>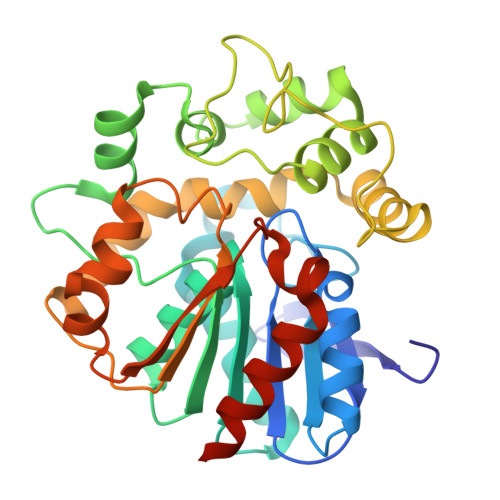 MEEIEHRTVEVNGIKMHVAEKGEGPVVLFLHGFPELWYSWRHQILALSSRGYRAVAPDLRGYGDTEAPVSISSYTGFHIVGDLIALIDLLGVDQVFLVAHDWGAIIGWYLCTFHPDRVKAYVCLSVPLLHRDPNIRTVDAMRAMYGDDYYICRFQKPGEMEAQMAEVGTEYVLKNILTTRKPGPPIFPKGEYGTGFNPDMPNSLPSWLTQDDLAYYVSKYEKTGFTGPLNYYRNMNLNWELTAPWSGGKIQVPVKFITGELDWVYTSLNMKEYIHGGGFKQDVPNLEEVIVQKNVAHFNNQEAAEEINNHIYDFIKKFLEHHHHHH>[2x]MAHHHHHHKQNEGIDVKKQENFSEWYSQVITKSEFLDYYDVSGCYIFRPNCWFVWESVQKFFDAEIKKLGVQNVMFPLFVTKRALETEKDHVEGFSPEVAWVTKSGNSDLQEPIALRPTSETIMYPSYAKWIQSHRDLPLKLNQWTNVVRWEFKHAVPFIRSREFYWQEGHSAFKSKEEADEEVFTILELYKRVYEELLAVPVIKGTKTENEKFAGADYTTTVETFIATNGRAVQGGTSHHL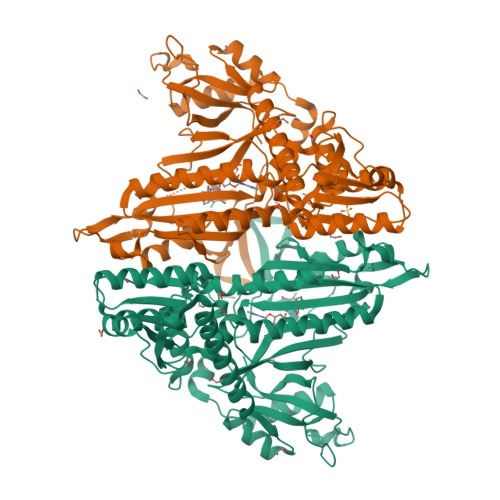GQNFSKMFKIQFEAENKETQFAYQNSWGLSTRTLGVMIMVHGDDKGMVLPPRVAFCQVVVIPLIFKDKDNATLVEKTKEIYNELEKAGIRVKLDDRLERTPGWKYNYWELRGVPLRIEVGPKDLEKQQIMLCRRDTGEKWTMPLSEFSGDSIKAVLDKIHDSMLNKARKEMNERIVVTRTWPEFIKALNSGNMCLIPWHESKAAEEYIKEKSKLESVQSQSDANTGLTGAAKSLCVPLDQSSFPSLEGLENFYPEEAHKKPNCWALFGRSY Herein, we report the first structural and kinetic characterization of a novel alkyl diamine N-hydroxylase DesB from Streptomyces sviceus (SsDesB). This enzyme catalyzes the first committed step in the biosynthesis of desferrioxamine B, a clinical drug used to treat iron overload disorders. Using the electron donor NADPH and molecular oxygen, NMOs catalyze the first committed step in hydroxamate siderophore biosynthesis by oxidizing a primary amine in alkyl amines and amino acids, such as lysine and ornithine, to N-hydroxylated products. SsDesB crystallized as a homotetramer with each protomer consisting of two dinucleotide-binding Rossman-fold domains: an FAD-binding domain (red) and an NADPH-binding domain (blue).

In the SsDesB-FAD complex structure, the FAD molecule is bound in an elongated conformation with the fully planar isoalloxazine ring positioned at the interface of the two dinucleotide-binding domains and a large area of the molecule, particularly the adenine dinucleotide portion, is exposed to solvent. In the holoenzyme, FAD is held in the active site pocket primarily by hydrogen bonding interactions involving S43, E42, K44, H50, P390, and W49 along the flavin adenine nucleotide backbone while residues Q61 and L392 contribute direct hydrogen bonds to the planar isoalloxazine ring primarily via the backbone amide nitrogen atoms. For our crystallization efforts, we used concentrated protein eluted from an IMAC column in which the aliquots retained a deep yellow color. However, similar crystallization hits could also be obtained after adding exogenous FAD to the protein aliquots after passage through a size exclusion column and then concentrating the protein. The fit of the FAD molecule to the final 2Fo-Fc electron density map (blue mesh, 2.86 Å resolution, contoured at 1σ level) is shown. The SsDesB active site appears to be more solvent exposed, which may contribute to its uncoupled mechanism as a lower amount of FAD copurified with the enzyme compared to that of other N-hydroxylases (75% flavin in NbtG and 50–60% flavin in SidA) in which FAD is buried and inaccessible by solvent.

>MTARPENPSTVHDFVGIGLGPFNLGLACLTEPIDELDGIFLESKPDFEWHAGMFLDGAHLQTPFMSDLVTLADPTSPYSFLNYLKEKGRLYSFYIRENFYPLRVEYDDYCRWAANKLSSIRFGTTVTEVRYEDDLYVVTTSAGDVYRARHLVLGTGTPPYIPEACQGLDGDFIHNSRYVQHRSELVKKESITIVGSGQSAAEIYQDLLGEIDVHGYRLNWVTRSPRFFPLEYTKLTLEMTSPEYIDYYRELPEATRYRLTAEQKGLFKGIDGDLINEIFDLLYQKNLAGPVPTRLLTNSSLNSARHENGTYTLAFRQEEQGKDFEIESQGLVLATGYKYAEPEFLAPVKDRLVYDSQGNFDVSRAYAIDVTGRGVFLQNAGVHTHSITSPDLGMGAYRNSCIIRELLGTEYYPVEKTIAFQEFSV[8x]>LFIEW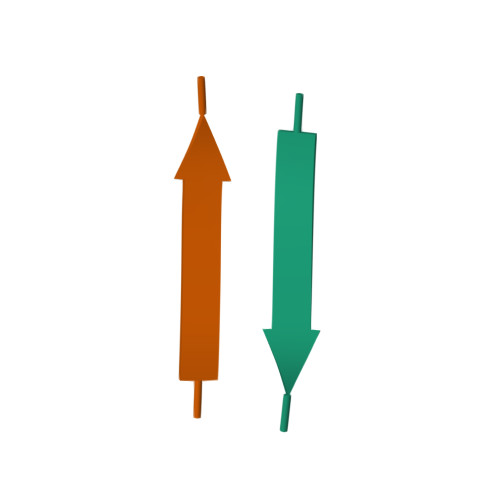L[4x]> GMQSWSAPAIPVVPGRGPALRLFDSADRQVRPVTPGPTATMYVCGITPYDATHLGHAATYLTFDLVHRLWLDAGHTVQYVQNVTDVDDPLFERAERDGIDWRTLGDRETQLFREDMAALRVLPPHDYVAATDAIAEVVEMVEKLLASGAAYIVEDAEYPDVYFRADATAQFGYESGYDRDTMLTLFAERGGDPDRPGKSDQLDALLWRAERPGEPSWPSPFGRGRPGWHVECSAIALTRIGTGLDIQGGGSDLIFPHHEYSAAHAESVTGERRFARHYVHTGMIGWDGHKMSKSRGNLVLVSQLRAQGVDPSAIRLGLFSGHYREDRFWSNEVLDEANARLARWRSATALPEAPDATDVIARVRQYLADDLDTPKALAALDGWCTDALSYGGHDTESPRLVATTVDALLGVDL

MshC catalyzes the ATP-dependent ligation of 1-O-(2-amino-2-deoxy-α-d-glucopyranosyl)-d-myo-inositol (GlcN-Ins) with l-cysteine (l-Cys) to form l-Cys-GlcN-Ins, the penultimate step in MSH biosynthesis. Mycothiol (MSH), the major cellular thiol in Mycobacterium tuberculosis (Mtb), plays an essential role in the resistance of Mtb to various antibiotics and oxidative stresses. Structurally, MshC is similar to class I aminoacyl-tRNA synthetases (aaRSs), especially to CysRS. We here opted for Ms-MshC to carry out affinity determination as the enzyme highly resembles Mtb-MshC with an overall sequence identity and similarity of 79% and 88%, respectively.

Therefore, a crystal structure of full-length MshC is required for a better understanding of the function of this enzyme and elucidation of the binding mechanism of MshC inhibitors. Here, we determined the crystal structure of the full-length Ms-MshC at 2.4 Å resolution. While the published MshC structure in complex with CSA contains two macromolecules in the asymmetric unit (ASU), all structures solved in this work only possess one macromolecule per ASU despite crystalizing in two different space groups. At the same time, the α-helix containing residues P88–R95 is disordered in our apo structure, while it is fully structured in the CSA-bound structure. Detailed analysis of these two structures showed that CSA binding induces a shift of the T46-H52 loop region towards the active site, whereby the side chain of Y48 is flipped inwards into the binding pocket. This concerted conformational change avoids the steric clash between the side chain of Y48 in the apo structure and the ordered positioning of the P88–R95 containing α-helix upon CSA binding. Additionally, the full-length crystal structures of ligand-free and compound-bound MshC provide the first glimpse of how this sulfonamide scaffold induces a number of conformational changes in the protein upon binding in the catalytic site.>GSAHAINKAGSLRMQSYRLLAAVPLSEKDKPLIKEMEQTAFSAELTRAAERDGQLAQLQGLQDYWRNELIPALMRAQNRETVSADVSQF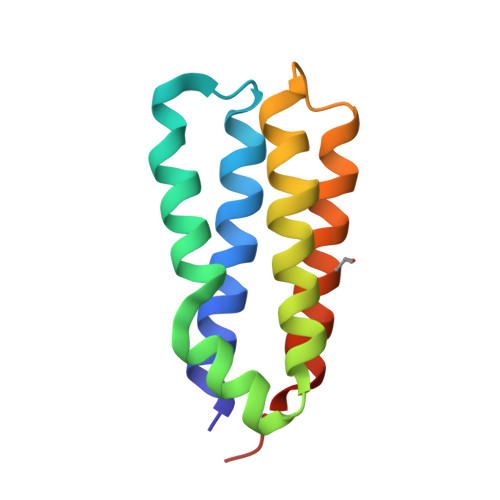VAGLDQLVSGFDRTTEMR[4x]>SWCLSVHQPWASLLVRGIKRVEGRSWYTPHRGRLWIAATAKKPSPQEVSELQATYRLLR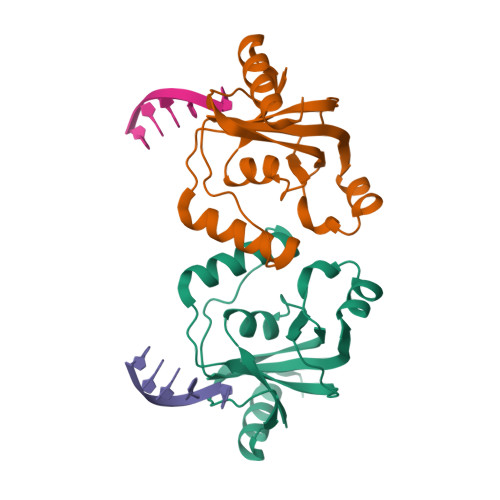GKDVEFPNDYPSGCLLGCVDLIDCLSQKQFKEQFPDISQESDSPFVFICKNPQEMVVKFPIKGNPKIWKLDSKIHQGAKKGLMKQNKAV[2x]>[2x]MRGVFLDKDKIPYDLVTKKLNEWYTSIKNDQVEQAEIIKTEVEKELLNMEENQDALLYYQLLEFRHEIMLSYMKSKEIEDLNNAYETIKEIEKQGQLTGMLEYYFYFFKGMYEFRRKELISAISAYRIAESKLSEVEDEIEKAEFFFKVSYVYYYMKQTYFSMNYANRALKIFREYEEYAVQTVRCQFIVAGNLIDSLEYERALEQFLKSLEISKESNIEHLIAMSHMNIGICYDELKEYKKASQHLILALEIFEKSKHSFLTKTLFTLTYVEAKQQNYNVALIYFRKGRFIADKSDDKEYSAKFKILEGLFFSDGETQLIKNAFSYLASRKMFADVENFSIEVADYFHEQGNLMLSNEYYRMSIEARRKIKKGEIIDENQPDSIGSSDFK

The large family of Gram-positive quorum-sensing receptors known as the RNPP proteins consists of receptors homologous to the Rap, NprR, PlcR, and PrgX proteins that are regulated by imported oligopeptide autoinducers. Rap proteins are phosphatases and transcriptional anti-activators, and NprR, PlcR, and PrgX proteins are DNA binding transcription factors. Rap proteins and their inhibitory oligopeptides, called Phr peptides, have been most extensively studied in B. subtilis, which encodes 11 Rap proteins on its chromosome and another five on plasmids. Sequence and structural analysis shows that the Rap proteins are repeat proteins consisting of nine HTH TPR or TPR-like folds, which pack together to form a right-handed superhelical TPR domain.

To reveal the structure of a Rap protein alone, we crystallized and determined the 2.44 Å resolution X-ray crystal structure of RapI. While discussed extensively below, it is worthwhile to note here that there are two copies of RapI in the crystallographic asymmetric unit, and while one model is relatively complete, there was in fact insufficient electron density to build helix-turn-helix (HTH) 1 and HTH2 in the second model (see Discussion and Materials and Methods). Similarly, comparing the structure of RapI with the structures of RapH-Spo0F and RapF-ComAC revealed that the RapI 3-helix bundle and linker region have joined the TPR domain; however, it is important to note that RapI and RapJ are not in identical conformations. The RapI structure reflects this scenario, and the ligand-binding groove is in an open conformation. Therefore, we evaluated the ability of RapI to dephosphorylate Spo0F in vitro, and we found that RapI is indeed a Spo0F phosphatase. Furthermore, we determined that the pentapeptide DRVGA and hexapeptide ADRVGA, sequences derived from the pro-PhrI C-terminus, inhibit RapI phosphatase activity in vitro. In the more complete RapI model, where the N-terminal 3-helix bundle and linker region are included, the N-terminal 3-helix bundle, linker region, and C-terminal TPR domain together bury 857 Å2 surface area at their interface. However, consistent with the idea that the structure of RapI depicts one of many transient conformations, we note that the position of the N-terminal 3-helix bundle and linker region in the more complete RapI model is likely influenced by crystal contacts with symmetry-related copies of RapI. More likely is the possibility that the structure of RapI alone depicts one of many transient conformations that the 3-helix bundle and linker region can adopt in the absence of a Phr peptide or target protein. In comparison to the Spo0F and ComAC bound structures, in both the RapI and RapJ-PhrC structures, the N-terminal 3-helix bundle has rotated ∼180° and the linker region helix has rotated ∼135°.> VATQPAPLYPDVGQDEAEKLGFEKVSE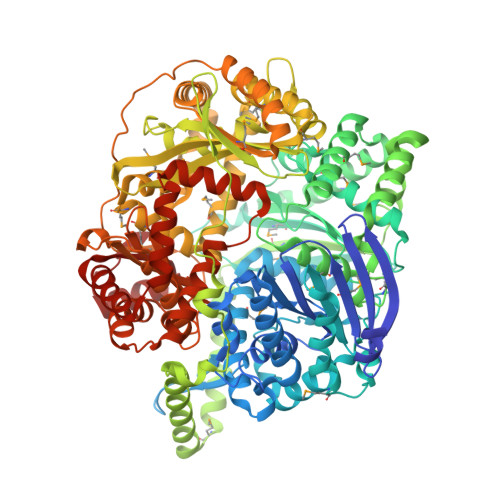EFISECKSKAILFKHKKTGCEVMSVSNEDENKVFGVVFRTPPKDSTGIPHILQHSVLCGSRKYPVKEPFVELLKGSLHTFLNAFTYPDRTCYPVASTNTKDFYNLVDVYLDAVFFPKCVDDAHTFQQEGWHYELNDPSEDISYKGVVFNEMKGVYSQPDNILGRIAQQALSPENTYGVDSGGDPKDIPNLTFEEFKEFHRQYYHPSNARIWFYGDDDPVHRLRVLSEYLDMFEASPSPNSSKIKFQKLFSEPVRLVEKYPAGRDGDLKKKHMLCVNWLLSEKPLDLQTQLALGFLDHLMLGTPASPLRKILLESGLGEALVSSGLSDELLQPQFGIGLKGVSEENVQKVEELIMDTLKKLAEEGFDNDAVEASMNTIEFSLRENNTGSFPRGLSLMLQSISKWIYDMDPFEPLKYTEPLKALKTRIAEEGSKAVFSPLIEKLILNNSHRVTIEMQPDPEKATQEEVEEKNILEKVKAAMTEEDLAELARATEELKLKQETPDPPEALRCVPSLNLGDIPKEPTYVPTEVGDINGVKVLRHDLFTNDIIYTEVVFDIGSLKHELLPLVPLFCQSLLEMGTKDLTFVQLNQLIGRKTGGISVYPLTSSVRGKDEPCSKIIVRGKSMAGRADDLFNLMNCLLQEVQFTDQQRFKQFVSQSRARMENRLRGSGHGIAAARMDAMLNIAGWMSEQMGGLSYLEFLHTLEKKVDEDWEGISSSLEEIRRSLLARNGCIVNMTADGKSLTNVEKSVAKFLDLLPENPSGGLVTWDGRLPLRNEAIVIPTQVNYVGKAGNIYSTGYELDGSAYVISKHISNTWLWDRVRVSGGAYGGFCDFDSHSGVFSYLSYRDPNLLKTLDIYDGTGDFLRGLDVDQETLTKAIIGTIGDVDSYQLPDAKGYSSLLRHLLGVTDEERQRKREEILTTSLKDFKDFAQAIDVVRDKGVAVAVASAEDIDAANNERSNFFEVKKAL>[3x]GMERAAFGKLVQALRREHRDEKGRVWTQEVLAERTQLPKRTIERIENGSLAHLDADILLRLADALELTIGERREF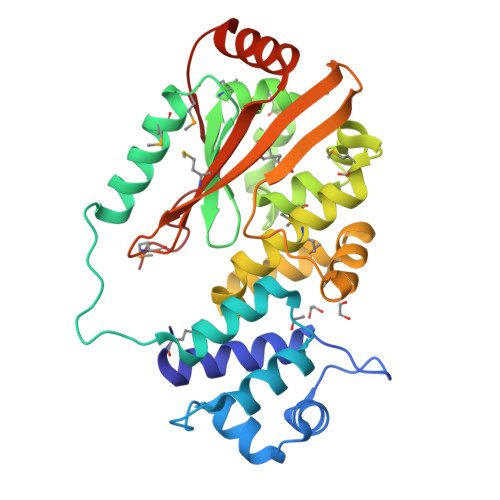FFAATGIIEQKSATYKRSPEESLQYLIDMIRNMNVPAFVTDQYVNIIAANMITIRFFNIPMELIETAPLLPHGYNLMRVVFGTEYDFRRVVGTMWDEVARHNMQLFRAISLRVRADGYFVELLDNLMQYREFKRFWERAHLETEDTSAENFWYQYTHPVYGLLSYVSSRSQIPTSMGLLSMHTYIPLSPATTDLFAKLSTVANQDVIRLAPWPRSNG2-({3-[(3,5-dibromo-2-ethoxybenzyl)amino]propyl}amino)quinolin-4(1H)-one | C21 H23 Br2 N3 O2 | 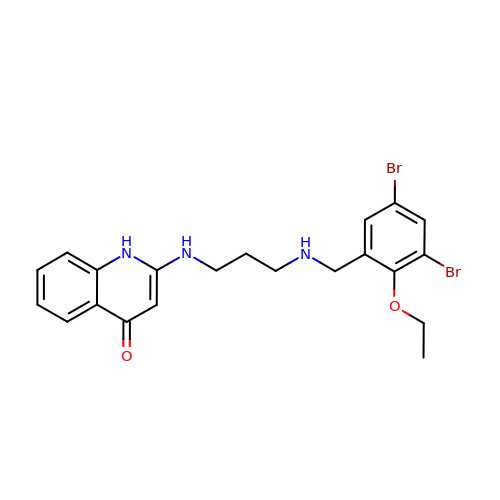IAGLKMDFSLVFID-UHFFFAOYSA-N>[3x]MKAIVVYLSTSGNTKAMAEAIGNGIESKNVDVQVISFYDVKLDELKEAEAIAVGSSTFYYK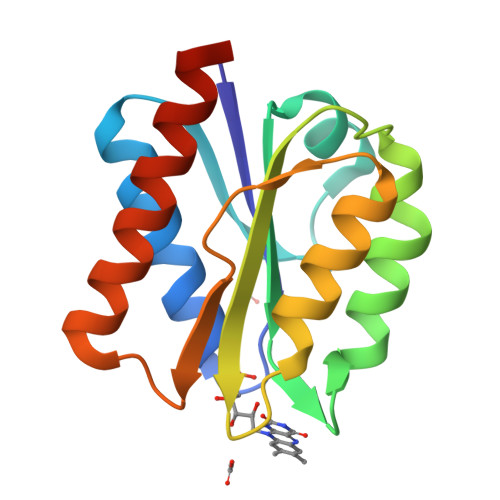MLLPMEKFMDETLVASNPQGKIGAAFGSYGWSGEAPILIAEKMREMGMTVMDPVLRILHKPTDKDLQECKRLGIDIAEKVKHKGTKAE> TNQHFVMVEVHRPDSEPDVNE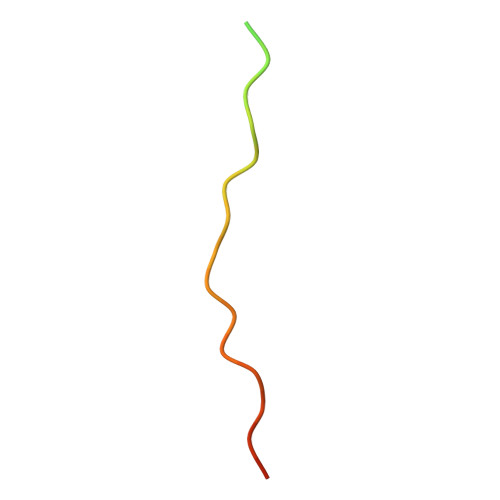VRALPQTRT N~4~-(3-methyl-1H-indazol-6-yl)-N~2~-(3,4,5-trimethoxyphenyl)pyrimidine-2,4-diamine 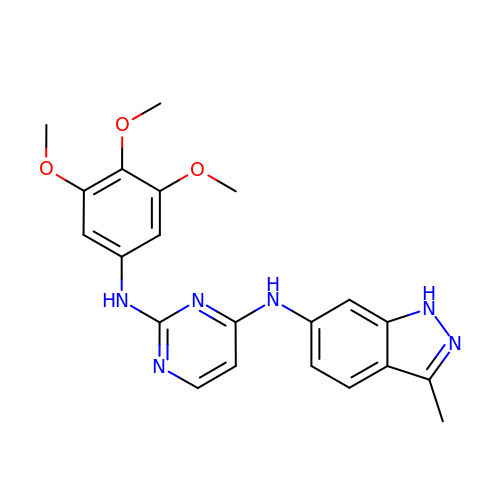| C21 H22 N6 O3 | SQQAPOSROFWHIB-UHFFFAOYSA-N> MEHRAFKWPQPLAGNKPRIWYGGDYNPDQWPEEVWDEDVALMQQAGVNLVSVAIFSWAKLEPEEGVYDFDWLDRVIDKLGKAGIAVDLASGTASPPMWMTQAHPEILWVDYRGDVCQPGARQHWRATSPVFLDYALNLCRKMAEHYKDNPYVVSWHVSNEYGCHNRFDYSEDAERAFQKWCEKKYGTIDAVNDAWGTAFWAQRMNNFSEIIPPRFIGDGNFMNPGKLLDWKRFSSDALLDFYKAERDALLEIAPKPQTTNFMVSAGCTVLDYDKWGHDVDFVSNDHYFSPGEAHFDEMAYAACLTDGIARKNPWFLMEHSTSAVNWRPTNYRLEPGELVRDSLAHLAMGADAICYFQWRQSKAGAEKWHSAMV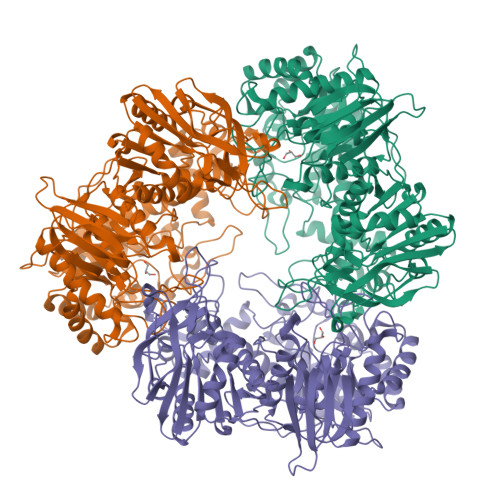PHAGPDSQIFRDVCELGADLNKLADEGLLSTKLVKSKVAIVFDYESQWATEHTATPTQEVRHWTEPLDWFRALADNGLTADVVPVRGPWDEYEAVVLPSLAILSEQTTRRVREYVANGGKLFVTYYTGLVDDRDHVWLGGYPGSIRDVVGVRVEEFAPMGTDAPGTMDHLDLDNGTVAHDFADVITSVADTAHVVASFKADKWTGFDGAPAITVNDFGDGKAAYVGARLGREGLAKSLPALLEELGIETSAEDDRGEVLRVERADETGENHFVFLFNRTHDVAVVDVEGEPLVASLAQVNESEHTAAIQPNGVLVVKLAAALEHHHHHH>MFKYLTPIFLCTAAISFQAQADDTMLMLLKKDNATYLSWSTDAGNVVRQDVYRSTSSAQAGSEKIAELNSSDRTFTDLTANPQSDYWYWVDTVSGNNSVLKSNAASTAPAPLRAAPLKAASPECKAGAVIKDKTVDCGGITLGLSCSGDSDKQPPVITLENATIKNLRISEKGGSDGIHCKSGNCRIENVIWED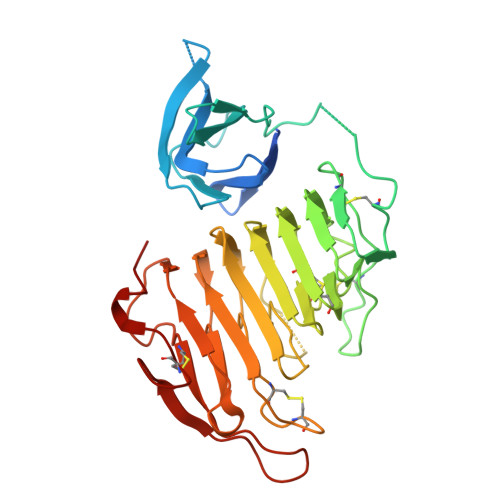ICEDAATNLGKTMTIVGGVAHNTTNGPGGKPDKVLQQNAKNSHTIVQGNFTLTGQHGKLWRSCGDCTNNGGPRNLTIISATVNGTIDSIAGVNRNFGDVAEIRDLRIKGYKEGKPPVCEEFNGVEKGKGKSDKYGEFWDTKNCKVSRSNVKPL[2x]> XSEAAAS;> LLF;>[2x]HGSPVDICTAKPRDIPMNPMCIYRSPEKKATEDEGSEQKIPEATNRRVWELSKANSRFATTFYQHLADSKNDNDNIFLSPLSISTAFA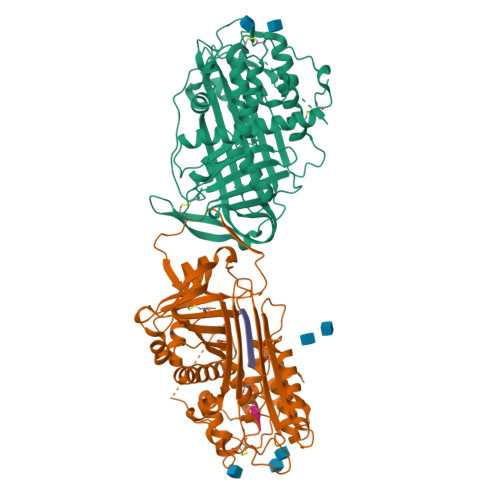MTKLGACNDTLQQLMEVFKFDTISEKTSDQIHFFFAKLNCRLYRKANKSSKLVSANRLFGDKSLTFNETYQDISELVYGAKLQPLDFKENAEQSRAAINKWVSNKTEGRITDVIPSEAINELTVLVLVNTIYFKGLWKSKFSPENTRKELFYKADGESCSASMMYQEGKFRYRRVAEGTQVLELPFKGDDITMVLILPKPEKSLAKVEKELTPEVLQEWLDELEEMMLVVHMPRFRIEDGFSLKEQLQDMGLVDLFSPEKSKLPGIVAEGRDDLYVSDAFHKAFLEVNEEGSEAAASTAVVIAGRSLNPNRVTFKANRPFLVFIREVPLNTIIFMGRVANPCVK> MAQTQGTRRKVCYYYDGDVGNYYYGQGHPMKPHRIRMTHNLLLNYGLYRKMEIYRPHKANAEEMTKYHSDDYIKFLRSIRPDNMSEYSKQMQRFNVGEDCPVFDGLFEFCQLSTGGSVASAVKLNKQQTDIAVNWAGGLHHAKKSEASGFCYVNDIVLAILELLKYHQRVLYIDIDIHHGDGVEEAFYTTDRVMTVSFHKYGEYFPGTGDLRDIGAGKGKYYAVNYPLRDGIDDESYEAIFKPVMSKVMEMFQPSAVVLQCGSDSLSGDRLGCFNLTIKGHAKCVEFVKSFNLPMLMLGGGGYTIRNVARCWTYETAVALDTEIPNELPYNDYFEYFGPDFKLHISPSNMTNQNTN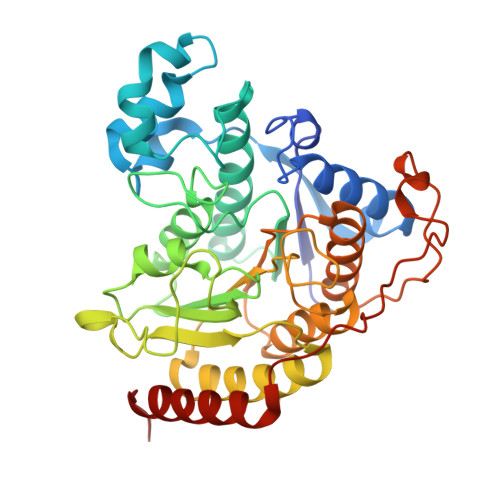EYLEKIKQRLFENLRMLPHA>GAHMAGRSMQAARCPTDELSLSNCAVVSEKDYQSGQHVIVRTSPNHKYIFTLRTHPSVVPGSVAFSLPQRKWAGLSIGQEIEVALYSFDKAKQCIGTMTIEIDFLQKKNIDSNPYDTDKMAAEFIQQFNNQAFSVGQQLVFSFNDKLFGLLVKDIEAMDPSILKGEPASGKRQKIEVGLVVGNSQVAFEKAENSSLNLIGKAKTKENRQSIINPDWNFEKMGIGGLDKEFSDIFRRAFASRVFPPEIVEQMGCKHVKGILLYGPPGCGKTLLARQIGKMLNAREPKVVNGPEILNKYVGESEANIRKLFADAEEEQRRLGANSGLHIIIFDEIDAICKQRGSMAGSTGVHDTVVNQLLSKIDGVEQLNNILVIGMTNRPDLIDEALLRPGRLEVKMEIGLPDEKGRLQILHIHTARMRGHQLLSADVDIKELAVETKNFSGAELEGLVRAAQSTAMNRHIKASTKVEVDMEKAESLQVTRGDFLASLEN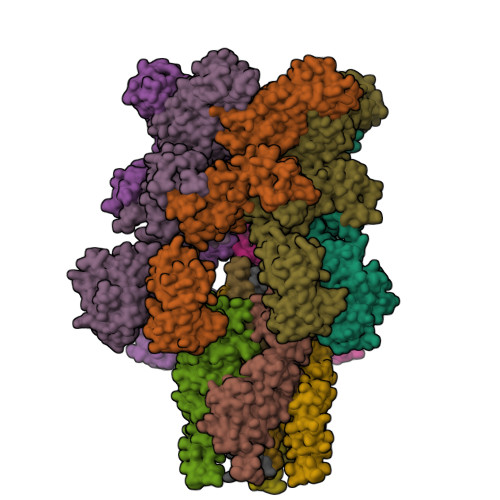DIKPAFGTNQEDYASYIMNGIIKWGDPVTRVLDDGELLVQQTKNSDRTPLVSVLLEGPPHSGKTALAAKIAEESNFPFIKICSPDKMIGFSETAKCQAMKKIFDDAYKSQLSCVVVDDIERLLDYVPIGPRFSNLVLQALLVLLKKAPPQGRKLLIIGTTSRKDVLQEMEMLNAFSTTIHVPNIATGEQLLEALELLGNFKDKERTTIAQQVKGKKVWIGIKKLLMLIEMSLQMDPEYRVRKFLALLREEGASPLDFD[6x];>GSMDTSGKQAEAMALLAEAERKVKNSQSFFSGLFGGSSKIEEACEIYARAANMFKMAKNWSAAGNAFCQAAQLHLQLQSKHDAATCFVDAGNAFKKADPQEAINCLMRAIEIYTDMGRFTIAAKHHISIAEIYETELVDVEKAIAHYEQSADYYKGEESNSSANKCLLKVAGYAAQLEQYQKAIDIYEQVGTSAMDSPLLKYSAKDYFFKAALCHFCIDMLNAKLAVQKYEELFPAFSDSRECKLMKKLLEAHEEQNVDSYTESVKEYDSISRLDQWLTTMLLRIKKTIQGDEEDLR[4x];> GSNRRLQQTQAQVDEVVDIMRVNVDKVLERDQKLSELDDRADALQAGASQFETSAAKLKRKYW;> MALSEIETRHSEIIKLENSIRELHDMFMDMAMLVESQGEMIDRIEYNVEHAVDYVERAVSDTKKAVK;> MRNELEEMQRRADQLADESLESTRRMLQLVEESKDAGIRTLVMLDEQGEQLDRVEEGMNHINQDMKEAEKNLKDLGKFCGLCVCPCNKLKSSDAYKKAWGNNQDGVVASQPARVVDEREQMAISGGFIRRVTNDARENEMDENLEQVSGIIGNLRHMALDMGNEIDTQNRQIDRIMEKADSNKTRIDEANQRATKMLG> GGGHNVAWDYDNNVIRGVNLGGWFVLEPYMTPSLFEPFQNGNDQSGVPV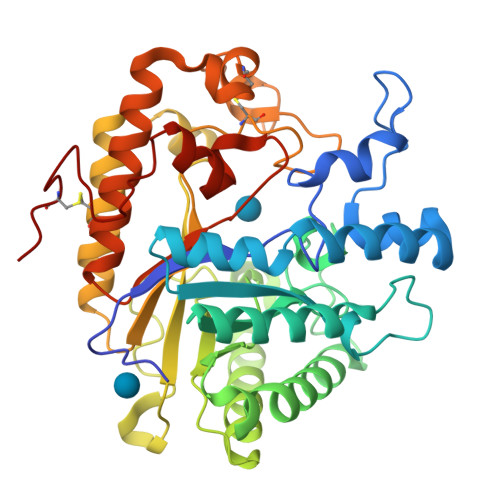DEYHWTQTLGKEAALRILQKHWSTWITEQDFKQISNLGLNFVRIPIGYWAFQLLDNDPYVQGQVQYLEKALGWARKNNIRVWIDLHGAPGSQNGFDNSGLRDSYNFQNGDNTQVTLNVLNTIFKKYGGNEYSDVVIGIELLNEPLGPVLNMDKLKQFFLDGYNSLRQTGSVTPVIIHDAFQVFGYWNNFLTVAEGQWNVVVDHHHYQVFSGGELSRNINDHISVACNWGWDAKKESHWNVAGQWSAALTDCAKWLNGVNRGARYEGAYDNAPYIGSCQPLLDISQWSDEHKTDTRRYIEAQLDAFEYTGGWVFWSWKTENAPEWSFQTLTYNGLFPQPVTDRQFPNQCGFH>[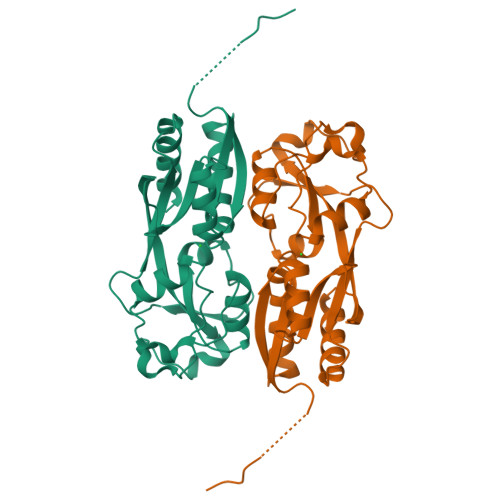2x]GAMELGSLCQGDSMQGQLKLGCIPTIAPFLLCDLVQEINQRFPQLNLLLREDTTTNLLTALRHGELDVLILALPVEIDGMESRVVGQDPFKMVISRHQAGAIKVPIKYDDLPDESVFLLEKEHCLTEHAVSACKLTDKEKINPFSATSLHTLVQMVANGLGTTFIPQMAIDHGLLDNQNLVVIEPPGQQAYRDIGLVWRPSSSRSKTFNQLAEVVSELL>LPVLAPVTKDPATSLYTIPFHDGASLVLDVAGPLVWSTCDGGQPPAEIPCSSPTCLLANAYPAPGCPAPSCGSDKHDKPCTAYPYNPVSGACAAGSLSHTRFVANTTDGSKPVSKVNVGVLAACAPSKLLASLPRGSTGVAGLANSGLALPAQVASAQKVANRFLLCLPTGGPGVAIFGGGPVPWPQFTQSMPYTPLVTKGGSPAHYISARSIVVGDTRVPVPEGALATGGVMLSTRLPYVLLRPDVYRPLMDAFTKALAAQHANGAPVARAVEAVAPFGVCYDTKTLGNNLGGYAVPNVQLGLDGGSDWTMTGKNSMVDVKQGTACVAFVEMKGVAAGDGRAPAVILGGAQMEDFVLDFDMEKKRLGFSRLPHFTGCGGL[2x];>SAG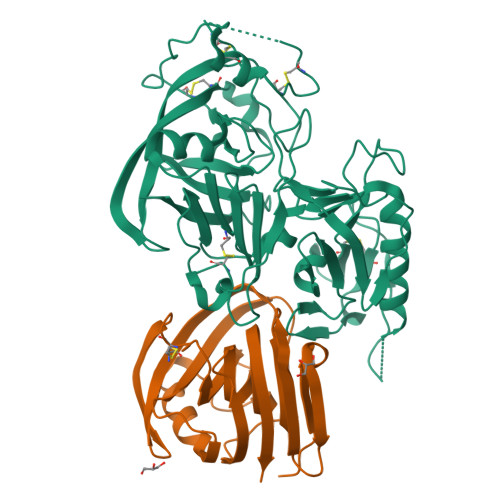INYVQNYNGNLGDFTYDESAGTFSMYWEDGVSSDFVVGLGWTTGSSNAITYSAEYSASGSSSYLAVYGWVNYPQAEYYIVEDYGDYNPCSSATSLGTVYSDGSTYQVCTDTRTNEPSITGTSTFTQYFSVRESTRTSGTVTVANHFNFWAQHGFGNSDFNYQVMAVEAWSGAGSASVTISS[2x]> EMETYVNKLHEGSTYTAAVQYNVLEKDDDPASLTIWVPMFQSSMPADLLIKELANVNILVKQISTPKGPSLRVM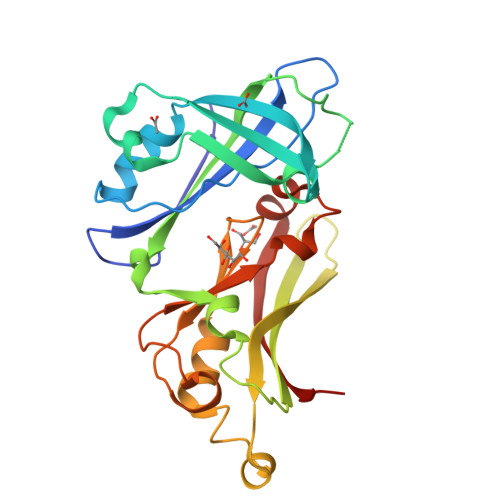INSRSAVLAQMPSKFTICANVSLDDRSKLAYDVTTPCEIKACSLTCLKSKNMLTTVKDLTMKTLNPTHDIIALCEFENIVTSKKVIIPTYLRSISVRNKDLNTLENITTTEFKNAITNAKIIPYSGLLLVITVTDNKGAFKYIKPQSQFIVDLGAYLEKESIYYVTTNWKHTATRFAIKPRED>ASAGVAVTNLNLKPGHCVEIKGSIPPDCKGFAVNLGEDASNFLLHFNARFDLHGDVNKIVCNSKEADAWGSEQREGVFPFQQGAEVMVCFEYQTDKIIIKFSSGDQFSFPVRKVLPSIPFLSLEGLQFKSITTE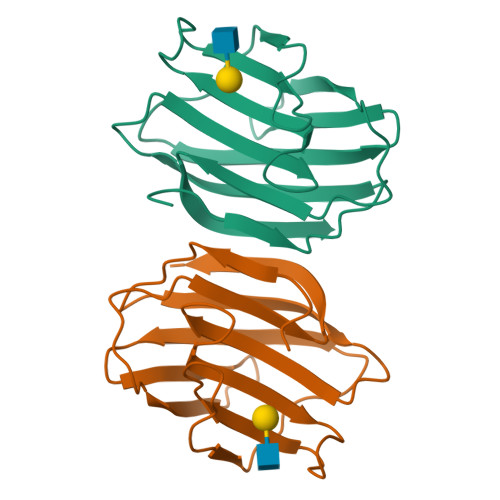[2x]> GSHMANPLAPYTLPQIATKVQVKHVPGKGRCLYTKHDLEPGSIIFVETPVLVAIPSLDEELWSVLTEINDEEALELPPVWHLAAICSLTMLDDEKKKICLDKWVPDPDRAPSDDVLRVINRAGLQVHPKLYERMLMVWRYNSFGHHTEQHGLVLYNRISMMAHSCRATACWHYGEDDAFILRARVKLQAGDELTISYIGDDDLFKSTNVRREKVYGWLFTCQCVRCAAPVDNARGFRCPLCGTGAMFFKTEDGETTSSACTICQAFPTQETIQEYLDFEQAYVDRLAETDKSDVPDAELVYNQATRVFAQHWVLYQLHTILFEGYRDAGNSESASFHQMERIKYVSQVMPLASYTLAWLYEEMGDTMLNKAEESGPEVPAHKLNVISRHFEDAYNLLYILCGEDHDYTVAAGTKKTACEERLP;> LAPYTLPQIATKVQVKHVPGKGRCLYTKHDLEPGSIIFVETPVLVAIPSLDEELWSVLTEINDEEALELPPVWHLAAICSLTMLDDEKKKICLDKWVPDPDRAPSDDVLRVINRAGLQVHPKLYERMLMVWRYNSFGHHTEQHGLVLYNRISMMAHSCRATACWHYGEDDAFILRARVKLQAGDELTISYIGDDDLFKSTNVRREKVYGWLFTCQCVRCAAPVDNARGFRCPLCGTGAMFFKTEDGETTSSACTICQAFPTQETIQEYLDFEQAYVDRLAETDKSDVPDAELVYNQATRVFAQHWVLYQLHTILFEGYRDAGNSESASFHQMERIKYVSQVMPLASYTLAWLYEEMGDTMLNKAEESGPEVPAHKLNVISRHFEDAYNLLYILCGEDHDYTVAAGTKKTACEERLPAS;> GSHMANPLAPYTLPQIATKVQVKHVPGKGRCLYTKHDLEPGSIIFVETPVLVAIPSLDEELWSVLTEINDEEALELPPVWHLAAICSLTMLDDEKKKICLDKWVPDPDRAPSDDVLRVINRAGLQVHPKLYERMLMVWRYNSFGHHTEQHGLVLYNRISMMAHSCRATACWHYGEDDAFILRARVKLQAGDELTISYIGDDDLFKSTNVRREKVYGWLFTCQCVRCAAPVDNARGFRCPLCGTGAM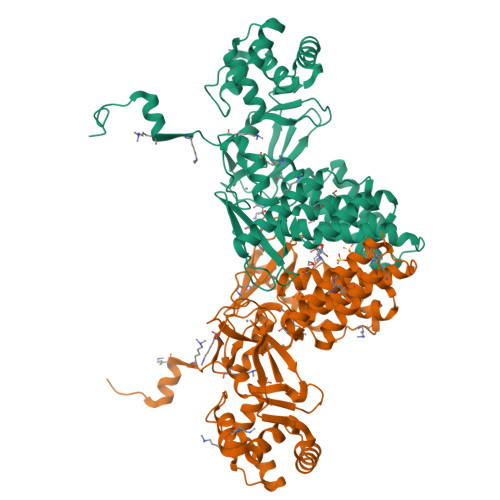FFKTEDGETTSSACTICQAFPTQETIQEYLDFEQAYVDRLAETDKSDVPDAELVYNQATRVFAQHWVLYQLHTILFEGYRDAGNSESASFHQMERIKYVSQVMPLASYTLAWLYEEMGDTMLNKAEESGPEVPAHKLNVISRHFEDAYNLLYILCGEDHDYTVAAGTKKTACEERLPA;> GSHMANPLAPYTLPQIATKVQVKHVPGKGRCLYTKHDLEPGSIIFVETPVLVAIPSLDEELWSVLTEINDEEALELPPVWHLAAICSLTMLDDEKKKICLDKWVPDPDRAPSDDVLRVINRAGLQVHPKLYERMLMVWRYNSFGHHTEQHGLVLYNRISMMAHSCRATACWHYGEDDAFILRARVKLQAGDELTISYIGDDDLFKSTNVRREKVYGWLFTCQCVRCAAPVDNARGFRCPLCGTGAMFFKTEDGETTSSACTICQAFPTQETIQEYLDFEQAYVDRLAETDKSDVPDAELVYNQATRVFAQHWVLYQLHTILFEGYRDAGNSESASFHQMERIKYVSQVMPLASYTLAWLYEEMGDTMLNKAEESGPEVPAHKLNVISRHFEDAYNLLYILCGEDHDYTVAAGTKKTACEERLPAS> GAHMDCHLSDMLQQLHSVNASKPSERGLVRQEEAEDPACIPIFWVSKWVDYSDKYGLGYQLCDNSVGVLFNDSTRLILYNDGDSLQYIERDGTESYLTVSSHPNSLMKKITLLKYFRNYMSEHLLKAGANITPREGDELARLPYLRTWFRTRSAIIL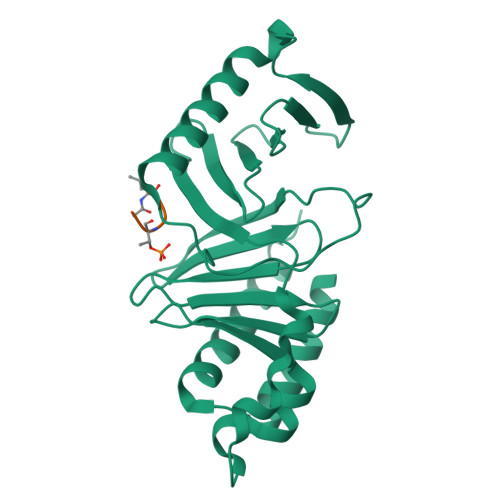HLSNGSVQINFFQDHTKLILCPLMAAVTYIDEKRDFRTYRLSLLEEYGCCKELASRLRYARTMVDKLLSSRSASNRLKA;> LHSTA> MNPIQKAWLKILEPVSYVINEKMAKRTGIIGKLGRFFAIGPREYGVHPINRMFIFMNRKYMAFQAVALHRYSFVKSLTHNGFHMLRVFRHFAFVLPATVLAGLGLFVYWGDDNKCYSPDRFPYLKKRAGD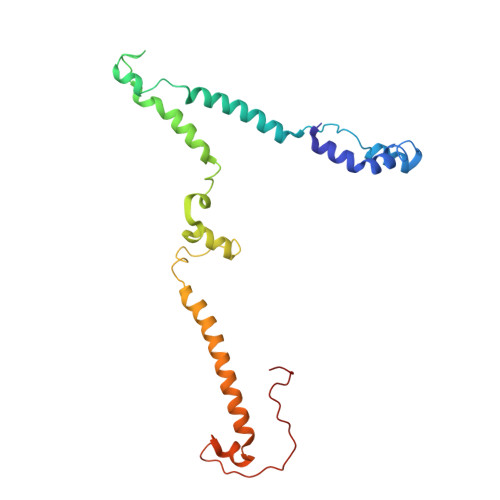MALPLNSLNQRTSAHYIEINAIYGAEMMKRYHKVWENIIEERSKATDQEKKTRYAHPSYQYSPLPVVSIPNVLNPLNLQ>[4x]SMQDPTIFEERHLKYISQLGKGNFGSVELCRYDPLGDNTGALVAVKQLQH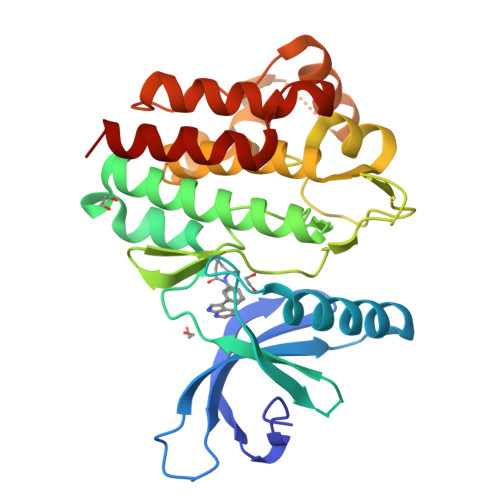SGPDQQRDFQREIQILKALHSDFIVKYRGVSYGPGRQSLRLVMEYLPSGCLRDFLQRHRARLDASRLLLYSSQICKGMEYLGSRRCVHRALAARNILVESEAHVKIADFGLAKLLPLDKDYYVVREPGQSPIFWYAPESLSDNIFSRQSDVWSFGVVLYELFTYCDKSCSPSAEFLRMMGSERDVPALSRLLELLEEGQRLPAPPACPAEVHELMKLCWAPSPQDRPSFSALGPQLDMLWSGSR>MLSRKGIIPEEYVLTRLAEDPTEPRYRTRERRARFVSKKGNCNVAHKNIREQGRFLQDVFTTLVDLKWPHTLLIFTMSFLCSWLLFAMVWWLIAFAHGDLAPGEGTNVPCVTSIHSFSSAFLFSIEVQVTIGFGGRMVTEECPLAILILIVQNIVGLMINAIMLGCIFMKTAQAHRRAETLIFSKHAVITLRHGRLCFMLRVGDLRKSMIISATIHMQVVRKTTSPEGEVVPLHQVDIPMENGVGGNSIFLVAPLIIYHVIDSNSPLYDLAPSDLHHHQDLEIIVILEGVVETTGITTQARTSYLADEILWGQRFVPIVAEEDGRYSVDYSKFGNTVKVPTPLCTARQLDEDRSLLDALTLASSRGPLRKRSVAVAKAKPKFSISPDSLS[4x];> MPLAFCGTENHSAAYRVDQGVLNNGCFVDALNVVPHVFLLFITFPILFIGWGSQSSKVHIHHSTWLHFPGHNLRWILTFILLFVLVCEIAEGILSDGVTESRHLHLYMPAGMAFMAAITSVVYYHNIETSNFPKLLIALLIYWTLAFITKTIKFVKFYDHAIGFSQLRFCLTGLLVILYGMLLLVEVNVIRVRRYIFFKTPREVKPPEDLQDLGVRFLQPFVNLLSKGTYWWMNAFIKTAHKKPIDLRAIAKLPIAMRALTNYQRLCVAFDAQARKDTQSPQGARAIWRALCHAFGRRLILSSTFRILADLLGFAGPLCIFGIVDHLGKENHVFQPKTQFLGVYFVSSQEFLGNAYVLAVLLFLALLLQRTFLQASYYVAIETGINLRGAIQTKIYNKIMHMSTSNLSMGEMTAGQICNLVAIDTNQLMWFFFLCPNLWTMPVQIIVGVILLYYILGVSALIGAAVIILLAPVQYFVATKLSQAQRTTLEHSNERLKQTNEMLRGMKLLKLYAWESIFCSRVEVTRRKEMTSLRAFAVYTSISIFMNTAIPIAAVLITFVGHVSFFKESDLSPSVAFASLSLFHILVTPLFLLSSVVRSTVKALVSVQKLSEFLSSAEIREEQCAPREP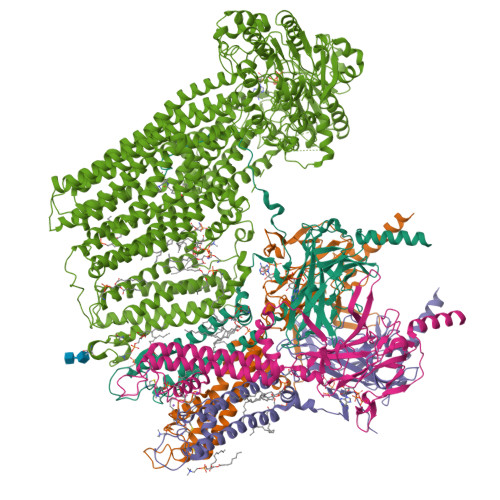APQGQAGKYQAVPLKVVNRKRPAREEVRDLLGPLQRLAPSMDGDADNFCVQIIGGFFTWTPDGIPTLSNITIRIPRGQLTMIVGQVGCGKSSLLLATLGEMQKVSGAVFWNSNLPDSEGEDPSSPERETAAGSDIRSRGPVAYASQKPWLLNATVEENITFESPFNKQRYKMVIEACSLQPDIDILPHGDQTQIGERGINLSGGQRQRISVARALYQQTNVVFLDDPFSALDVHLSDHLMQAGILELLRDDKRTVVLVTHKLQYLPHADWIIAMKDGTIQREGTLKDFQRSECQLFEHWKTLMNRQDQELEKETVMERKASEPSQGLPRAMSSRDGLLLDEEEEEEEAAESEEDDNLSSVLHQRAKIPWRACTKYLSSAGILLLSLLVFSQLLKHMVLVAIDYWLAKWTDSALVLSPAARNCSLSQECDLDQSVYAMVFTLLCSLGIVLCLVTSVTVEWTGLKVAKRLHRSLLNRIILAPMRFFETTPLGSILNRFSSDCNTIDQHIPSTLECLSRSTLLCVSALTVISYVTPVFLVALLPLAVVCYFIQKYFRVASRDLQQLDDTTQLPLVSHFAETVEGLTTIRAFRYEARFQQKLLEYTDSNNIASLFLTAANRWLEVCMEYIGACVVLIAAATSISNSLHRELSAGLVGLGLTYALMVSNYLNWMVRNLADMEIQLGAVKRIHALLKTEAESYEGLLAPSLIPKNWPDQGKIQIQNLSVRYDSSLKPVLKHVNTLISPGQKIGICGRTGSGKSSFSLAFFRMVDMFEGRIIIDGIDIAKLPLHTLRSRLSIILQDPVLFSGTIRFNLDPEKKCSDSTLWEALEIAQLKLVVKALPGGLDAIITEGGENFSQGQRQLFCLARAFVRKTSIFIMDEATASIDMATENILQKVVMTAFADRTVVTIAHRVHTILSADLVMVLKRGAILEFDKPETLLSQKDSVFASFVRADK> SNAETIEIIKDLFEHLCGVRVHRTYEDDTGLWFDTSQGSKNGIMDYKLGFVKSQAENTTEVDTEVIYVPLLKQRTAE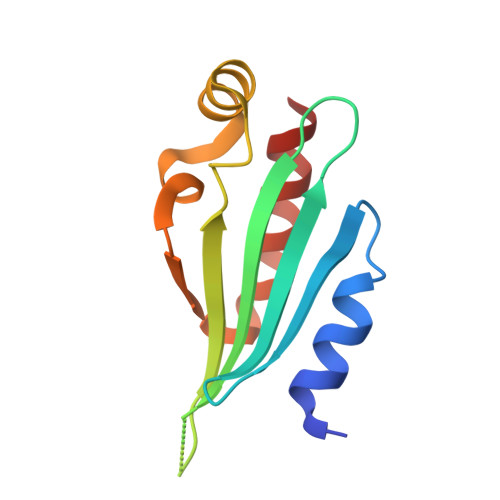ELQELQKKLPDYLFETLSFPLRSLNQFYIKMSKSLNKKV>AECSVDIQGNDQMQFNTNAITVDKSCKQFTVNLSHPGNLPKCVMGHNWVLSTAADMQGVVTDGEASGLDK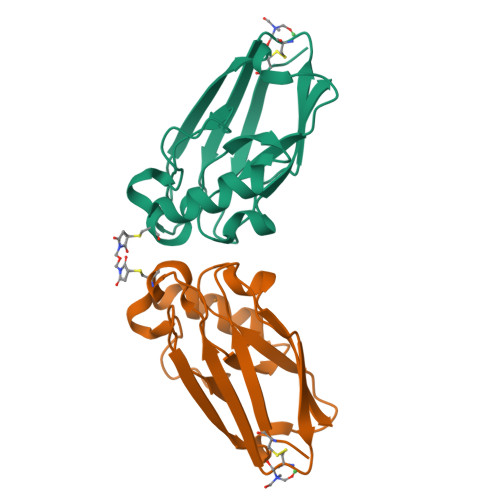DYLKPDDSRVIAHTKLIGSGEKDSVTFDVSKLKEGEQYMFFCTFPGHSALMKGTLTLK[2x]(6R)-2-amino-6-[2-(3'-methoxybiphenyl-3-yl)ethyl]-3,6-dimethyl-5,6-dihydropyrimidin-4(3H)-one | C21 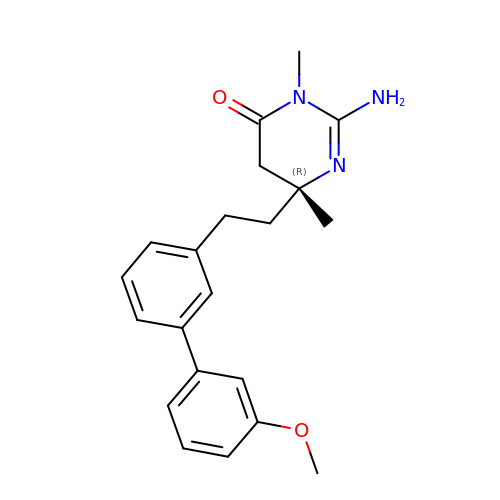H25 N3 O2 | VDFBMQAUECXNKR-OAQYLSRUSA-N>[4x]TNMSIKEQRESLPVFQFRDQIIQAVKDNQILIVVGETGSGKTTQ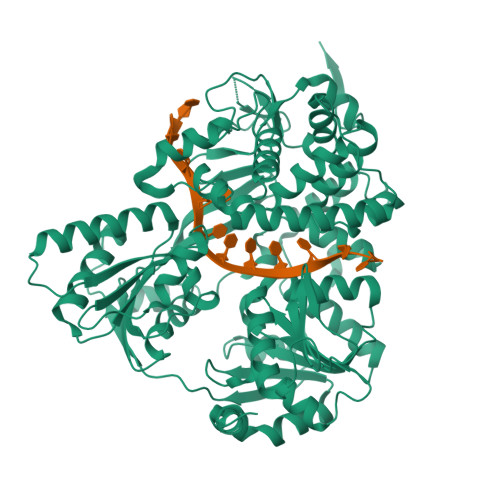VTQYLAEAGFTKYGMIGCTQPRRVAAVSVAKRVAEEVGCQLGQEVGYTIRFEDVTSPATKIKYMTDGMLQREILMDPDLKRYSVIMLDEAHERTIATDVLFALLKKTVKRRPDLKVIVTSATLDAEKFSEYFNSCPIFTIPGRTFPVEILYSREPEPDYLEAALTTVMQIHLTEPPGDILVFLTGQEEIDTACEILYERMKALGPSVPELIILPIYSALPSEMQSRIFEPAPPGSRKVVIATNIAETAITIDYIYYVVDPGFVKQNAYDPKLGMDSLVVTPISQAQANQRAGRAGRTGPGKCFRLYTEAAYQSEMLPTTIPDIQRQNLANTILLLKAMGINDLLRFDFMDPPPVNTMLTALEELYALGALDDEGLLTRLGRKMADFPMEPSLSKVLIASVDKGCSDEMVTIVSMLNLQQIFYRPKDKQQQADQKKAKFHDPTGDHLTLLNVYNAWKNSGYSNAWCFENYIQARAMRRARDVRQQIVKIMERHRHPIISCGRDTDKIRQALCAGFFRNTARKDPQEGYKTLTEGTPVYLHPSSALFGKQAEWVLYHELVLTTKEYMHFTTAIEPKWLVEAAPTFFKLAPTDRLSKRKKAERIQPLYNKYEGEDGWRLSAQRRAARPGGGGGTWG>MPGSIPLIGERFPEMEVTTDHGVIKLPDHYVSQGKWFVLFSHPADFTPVCTTEFVSFARRYEDFQRLGVDLIGLSVDSVFSHIKWKEWIERHIGVRIPFPIIADPQGTVARRLGLLHAESATHTVRGVF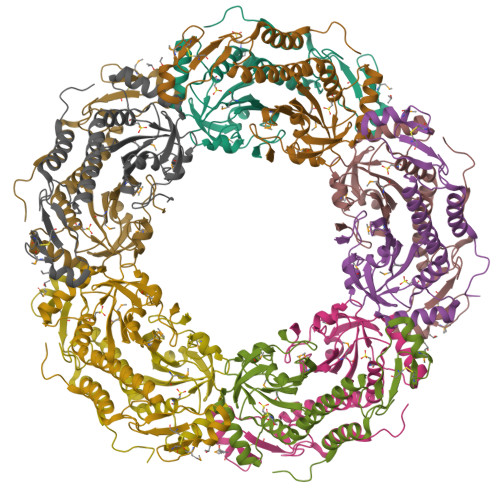IVDARGVIRTMLYYPMELGRLVDEILRIVKALKLGDSLKRAVPADWPNNEIIGEGLIVPPPTTEDQARARMESGQYRCLDWWFCWDTPASRDDVEEARRYLRRAAEKPAKLLYEEARTHLH[10x]>ENSVHRYKKEASNLIKLATPVLIASVAQTGMGFVDTIMAGGVSAIDMAAVSIAASIWLPSILFGVGLLMALVPVVAQLNGAGRQHKIPFEVHQGLILALLVSVPIIAVLFQTQFIIRFMDVEEAMATKTVGYMHAVIFAVPAYLLFQALRSFTDGMSLTKPAMVIGFIGLLLNIPLNWIFVYGKFGAPELGGVGCGVATAIVYWIMLLLLLFYIVTSKRLAHVKVFETFHKPQPKELIRLFRLGFPVAAALFFEVTLFAVVALLVAPLGSTVVAAHQVALNFSSLVFMFPMSIGAAVSIRVGHKLGEQDTKGAAIAANVGLMTGLATACITALLTVLFREQIALLYTENQVVVALAMQLLLFAAIYQCMDAVQVVAAGSLRGYKDMTAIFHRTFISYWVLGLPTGYILGMTNWLTEQPLGAKGFWLGFIIGLSAAALMLGQRLYWLQKQSDDVQLHLAAK[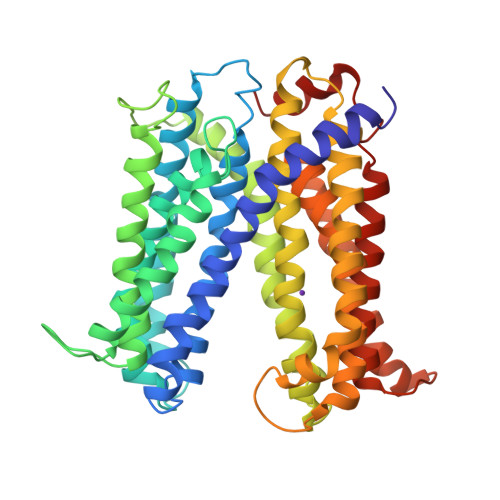2x]>[2x]MTQFTDIDKLAVSTIRILAVDTVSKANSGHPGAPLGMAPAAHVLWSQMRMNPTNPDWINRDRFVLSNGHAVALLYSMLHLTGYDLSIEDLKQFRQLGSRTPGHPEFELPGVEVTTGPLGQGISNAVGMAMAQANLAATYNKPGFTLSDNYTYVFLGDGCLQEGISSEASSLAGHLKLGNLIAIYDDNKITIDGATSISFDEDVAKRYEAYGWEVLYVENGNEDLAGIAKAIAQAKLSKDKPTLIKMTTTIGYGSLHAGSHSVAGAPLKADDVKQLKSKFGFNPDKSFVVPQEVYDHYQKTILKPGVEANNKWNKLFSEYQKKFPELGAELARRLSGQLPANWESKLPT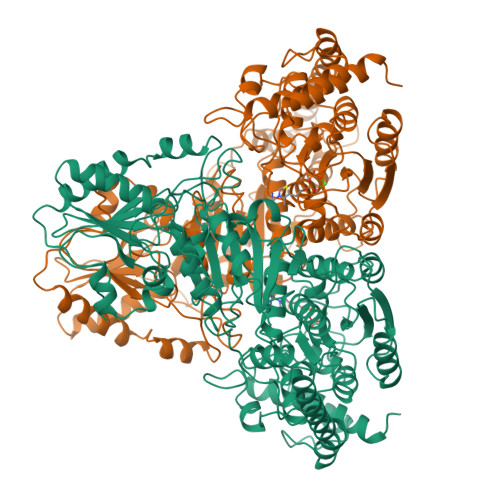YTAKDSAVATRKLSETVLEDVYNQLPELIGGSADLTPSNLTRWKEALDFQPPSSGSGNYSGRYIRYGIREHAMGAIMNGISAFGANYKPYGGTFLNFVSYAAGAVRLSALSGHPVIWVATHDSIGVGEDGPTHQPIETLAHFRSLPNIQVWRPADGNEVSAAYKNSLESKHTPSIIALSRQNLPQLEGSSIESASKGGYVLQDVANPDIILVATGSEVSLSVEAAKTLAAKNIKARVVSLPDFFTFDKQPLEYRLSVLPDNVPIMSVEVLATTCWGKYAHQSFGIDRFGASGKAPEVFKFFGFTPEGVAERAQKTIAFYKGDKLISPLKKAF2-acetamido-2-deoxy-beta-D-mannopyranose | C8 H15 N O6 | 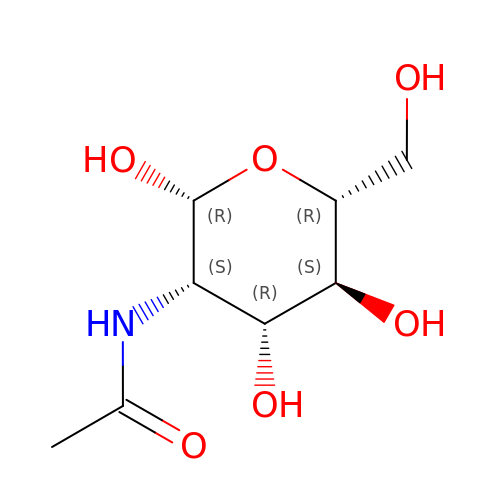OVRNDRQMDRJTHS-OZRXBMAMSA-N> MIEDPYLGKYVTCVSARSTDKEILKKAQDGGIATALMVYALEEGFIDGTIVAGEGDKPWQPKPVVAMTREDILKARGTRYNISPQISWLKEATRSFGLDKVGVTGVCCQMQAVRKAQLYPINMRDVPGKVAFTVGLFCMENFSYKSLQSIVEDHANQSLGSVKKMEITKGKFWVYTERGNVATVPLKATHKYEQPGCHVCLDYVSNLADISTGS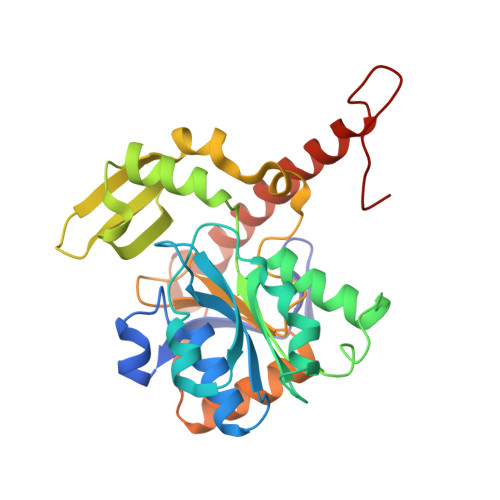VGSPDGWSTVFIRTKVGNEIWSKAVADGMFETKPIEEVKPGLDLLRKLAKQKIDKNQKTVEERKTFGINKGLRNPYA>MALKNTEIEVTGWEQALKWLRSNTSKYATATSWWDYGYWIESSLLGNRRASADGGHARDRDHILALFLARDGNISEVDFESWELNYFIIYLNDWAKFNAISYLGGAITRKEYNGDENGRGRVTTILLTQAAGNVYVNPYARIVIKVIQQNKTRRIAVNIGQLECSPILSVAFPGNIKIKGSGRCSDGSPFPYVVYLTPSLGVLAYYKVATSNFVKLAFGIPTSSYSEFAEKLFSNFIPVYQYGSVIVYEFRPFAI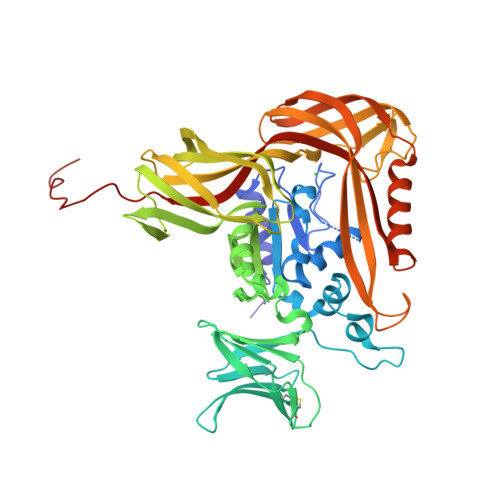YKIEDFINGTWREVGKLSPGKHTLRLYISAFGRDIKNATLYVYALNGTKIIKRIKVGEIKYMNHLEEYPIIVNVTLPTAQKYRFILAQKGPVGVLTGPVRVNGKITNPAYIMREGESGRLELKVGVDKEYTADLYLRATFIYLVRKGGKSNEDYDASFEPHMDTFFITKLKEGIKLRPGENEIVVNAEMPKNAISSYKEKLEKEHGDKLIIRGIRVEPVFIVEKEYTMIEVSASAPHHSSEHHHHHHHHHH[2x]>EVATYEDLISHKHDYPKEIYKESHYIRRNTRLDVIKKIPQFEQKSKEWLKQRTESLTATAISVVFDEDPYKHPIVILLDKCGRGLPFV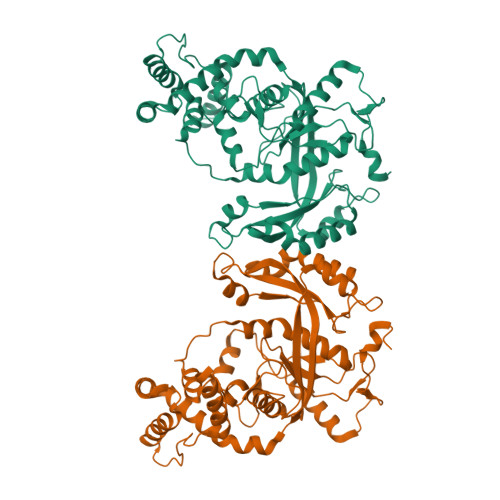ENKFVHHGNKYEQIGTMFYSFRNNVEVGEYGLLQHSGHKFIAASPDGICSKKANTGGLSKLVGRLLEIKFPFSREINNSGDLDGDICPHYYFLQVQTQLYVTEMDECDFLQCKIDEYDSWEDFVKDSNPIVPGLSKTTNLEKGCLIQLSDKNLIGSDDKEKCLYNSKYIYPPKLHMTNEEIEKWISSEIMNYHNNDLSENYMIDRVIYWRLSQVTCNLIKLNKEAFEEKIPLLQQFWDYVLFYRQHSDKLDKLIKFVEKVKEDNSAEIFSYINEDFLSLNKDSKYEPLYQEETEWRKKYNQIKAKKAQMYK[2x]> MKHHHHHHMTFPGDTAVLVLAAGPGTRMRSDTPKVLHTLAGRSMLSHVLHAIAKLAPQRLIVVLGHDHQRIAPLVGELADTLGRTIDVALQDRPLGTGHAV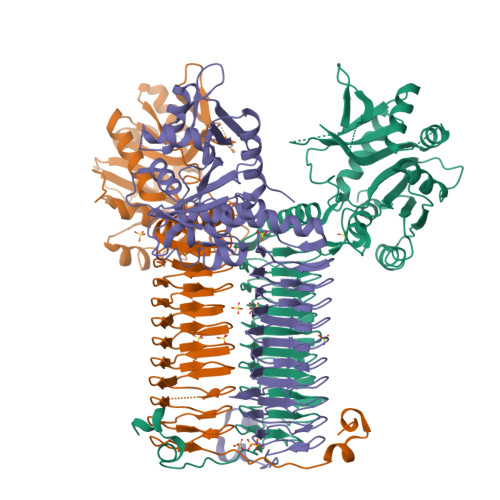LCGLSALPDDYAGNVVVTSGDTPLLDADTLADLIATHRAVSAAVTVLTTTLDDPFGYGRILRTQDHEVMAIVEQTDATPSQREIREVNAGVYAFDIAALRSALSRLSSNNAQQELYLTDVIAILRSDGQTVHASHVDDSALVAGVNNRVQLAELASELNRRVVAAHQLAGVTVVDPATTWIDVDVTIGRDTVIHPGTQLLGRTQIGGRCVVGPDTTLTDVAVGDGASVVRTHGSSSSIGDGAAVGPFTYLRPGTALGADGKLGAFVEVKNSTIGTGTKVPHLTYVGDADIGEYSNIGASSVFVNYDGTSKRRTTVGSHVRTGSDTMFVAPVTIGDGAYTGAGTVVREDVPPGALAVSAGPQRNIENWVQRKRPGSPAAQASKRASEMACQQPTQPPDADQTP> MPTVDDVLEQVGEFGWFQKQAFLTLCLLSAAFAPIYVGIVFLGFTPDHRCRSPGVAELSQRCGWSLAEELNYTVPGLGAAGEAFPRQCRRYEVDWNQSALSCVDPLASLAANRSHLPLGPCQHGWVYDTPGSSIVTEFNLVCADSWKVDLFQSCVNVGFFLGSLGVGYIADRFGRKLCLLATTLISAVSGVLMAVAPDYTSMLLFRLLQGLVSKGSWMSGYTLITEFVGSGYRRTVAILYQMAFTVGLVLLSGVAYAIPHWRWLQLAVSLPTFLFLLYYWCVPESPRWLLSQKRNTQAIKIMDHIAQKNGKLPPADLKMLSLKEDS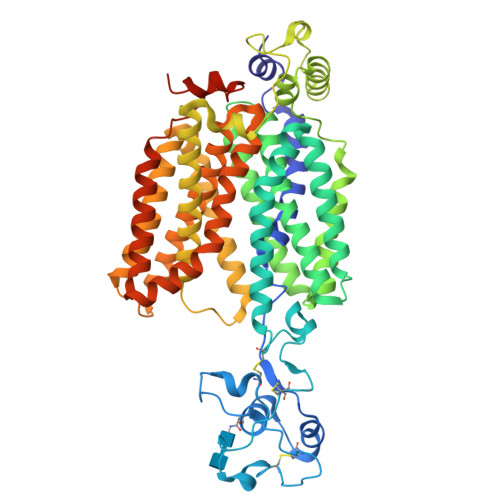TEKLSPSFADLFRTPQLRKHTFILMYLWFTSSVLYQGLIMHMGATGGNLYLDFFYSALVEFPAAFIILVTIDRVGRIYPLAVSNLVAGAACLIMIFISQDLHWLNITVACVGRMGITIVFQMVCLVNAELYPTFIRNLGVMVCSSLCDLGGIITPFLVFRLMEVWQGLPLILFTVVGLVAGGMTLLLPETKGVALPETIEDAENLGRKAKPKENTIYLQVQTSELPGT>[6x]GSSGSSGGTVKNYETAVQFCWNHYKDQMDPIEK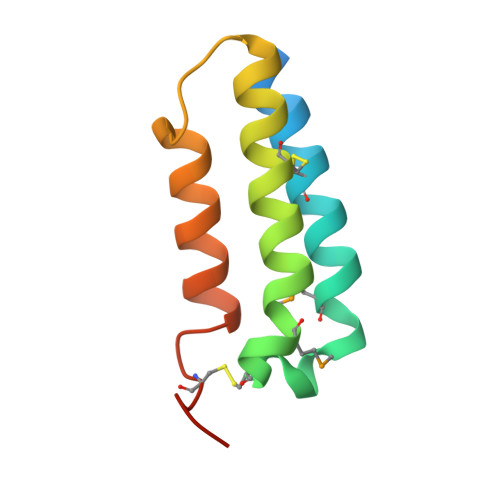DWCDWAMISRPYSTLRDCLEHFAELFDLGFPNPLAERIIFETHQIHFANCSLVQPTFS> AVISVKPILLAMTPVFILLCLFFGTR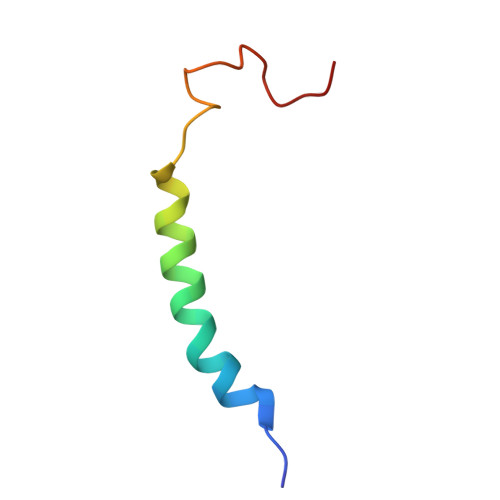NGFYDTDQYHGNAAAH> MAAPFDKSKNVAQSIDQLIGQTPALYLNKLNNTKAKVVLKMECENPMASVKDRLGFAIYDKAEKEGKLIPGKSIVVESSSGNTGVSLAHLGAIRGYKVIITMPESMSLERRCLLRIFGAEVILTPAALGMKGAVAMAKKIVAANPNAVLADQFATKYNALIHE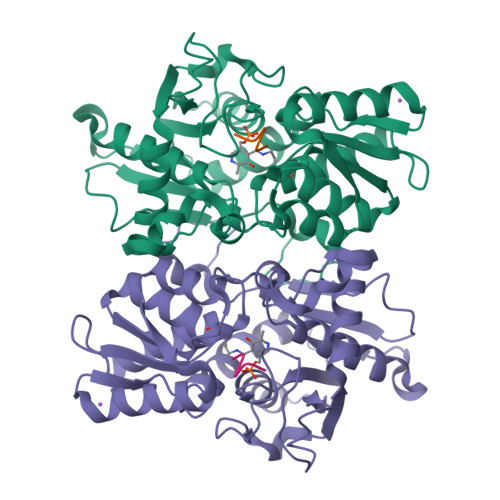ETTGPEIWEQTNHNVDCFIAGVGTGGTLTGVARALKKMGSHARIVAVEPTESPVLSGGKPGPHKIQGIGPGFVPDVLDRSLIDEVLCVAGDDAIETALKLTRSDGVFCGFSGGANVYAALKIAERPEMEGKTIVTVIPSFGERYLSTTLYRSVRDEVSSLPVALEHHHHHH;> LERDGSGI N-{3-[(1S,5S,6S)-3-amino-1-(methoxymethyl)-5-methyl-2-thia-4-azabicyclo[4.1.0]hept-3-en-5-yl]-4,5-difluorophenyl}-5-[(prop-2-yn-1-yl)oxy]pyrazine-2-carboxamide 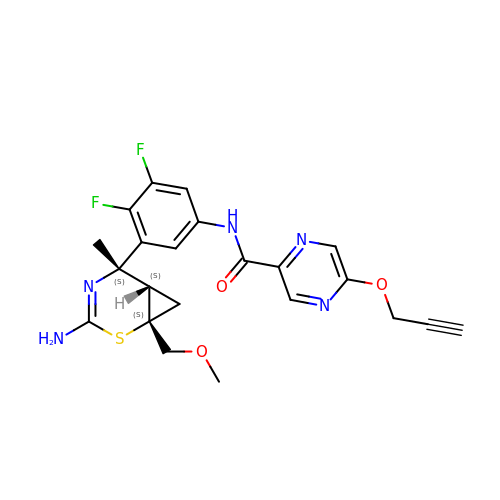| C22 H21 F2 N5 O3 S | IPUJINDWAGRAHN-KNXBSLHKSA-N>[2x]GSHMASREQTMENILKAAKKKFGERGYEGTSIQEIAKEAKVNVAMASYYFNGKENLYYEVFKKYGLANELPNFLEKNQFNPINALREY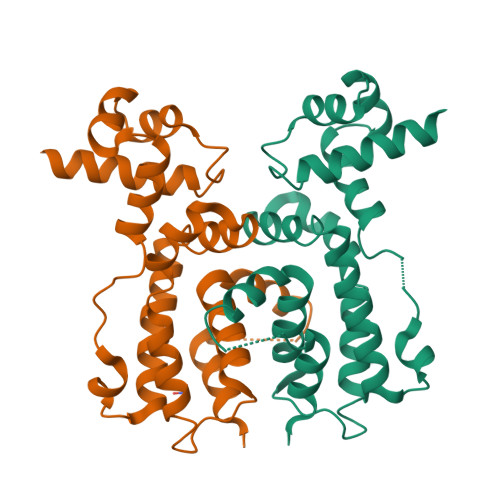LTVFTTHIKENPEIGTLAYEEIIKESARLEKIKPYFIGSFEQLKEILQEGEKQGVFHFFSINHTIHWITSIVLFPKFKKFIDGLVPRGSGGLVPRGSGDLVSRIISALTDKPNI Pyrrolysyl-tRNA synthetases (PylRSs) are naturally encoded in some archaeal and bacterial genomes to acylate tRNAPyl with pyrrolysine. Similar to the 20 canonical amino acids, Pyl also has a dedicated tRNA:aaRS pair (tRNAPyl:PylRS) for protein translation. To reveal the mechanism by which the Ma tRNAPyl identity elements mediate highly specific recognition of Ma tRNAPyl by MaPylRS, we determined two cryo-EM structures. We achieved high resolution (2.8–2.9Å) maps by using the ribosome as a scaffold for visualizing Ma or Mm tRNAPyl, a strategy that we previously showed to be successful.

Comparison of these two structures revealed four unique structural features of Ma tRNAPyl compared to Mm tRNAPyl, providing insight into its orthogonal recognition by MaPylRS. The first major difference is the absence of a base at position 8 (at the acceptor/D-stem junction). In Mm tRNAPyl, as in other tRNAs, the presence of U8 pushes G10 into a loop. Thirdly, Ma tRNAPyl has a pronounced C45 that is missing in the ribosome-bound Mm tRNAPyl. The reason for the difference in this region for Mm tRNAPyl is unclear, however we do know that position 45 is the first nucleotide in the variable arm. Previous studies have shown the importance of variable arm structure in the ribosome for efficient translation, and we know that in E. coli Mm tRNAPyl does not translate as well as Ma tRNAPyl. Finally, by overlaying the two tRNAPyl structures obtained from cryo-EM imaging on the ribosome, we found a nearly identical conformation of their acceptor stems and lower part of their anticodon stems (rmsd of 0.25–0.30 Å between their backbone atoms). However, the two tRNA structures began to deviate from each other (rmsd ∼1.5 Å between their backbone atoms) within a stretch between U8 and U28 in Mm tRNAPyl. This overall shape change appears to be caused by the elements in Ma tRNAPyl which we determined to be necessary for MaPylRS recognition; the deletion of U8 in Ma tRNAPyl truncating the loop between the acceptor stem and D-stem, and the mutation of U28:G42 to G28:U42 (and possibly the A42a intercalation) affecting the trajectory of the phosphate backbone. Starting with the pylSn-pylSc class of enzymes where the NTD is physically connected to the CTD with a linker, the cognate tRNA (Mm tRNAPyl) showed a high RMSF with an averaged structure that appeared like more of an obtuse angle than an L-shape.

> GGAAACCUGAUCAUGUAGAUCGAAUGGACUCUAAAUCCGUUCAGCCGGGUUAGAUUCCCGGGGUUUCCGCCA> DNLMERANSMFEPIPKYPPVIDGNELTQAKVELGKMEFFEPRLSSSHLISCNTCHNVGLGGDDELPTSIGHGWQKGPRNSPTVFNAVFNAAQFWDGRAADLAEQAKGPVQAGVEMSSTPDRVVATLKSMPEYIERFEDAFPGQENPVTFDNMAVAIEAYEATLITPEAPFDKYLRGDTSALNESEKEGLALFMDRGCTACHSGVNLGGQNYYPFGLVAKPGAEILPEGDKGRFSVTETASDEYVFRASPLRNIELTAPYFHSGAVWSLEEAVAVMGTAQLGTELNNDEVKSIVAFLKTLTGNVPEVTYPVLPPSTANTPKPVD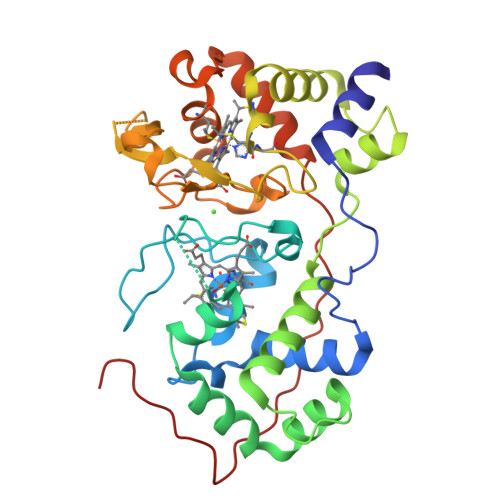MIP>[2x]GSHMDSKHQCVKLNDGHFMPVLGFGTYAPPEVP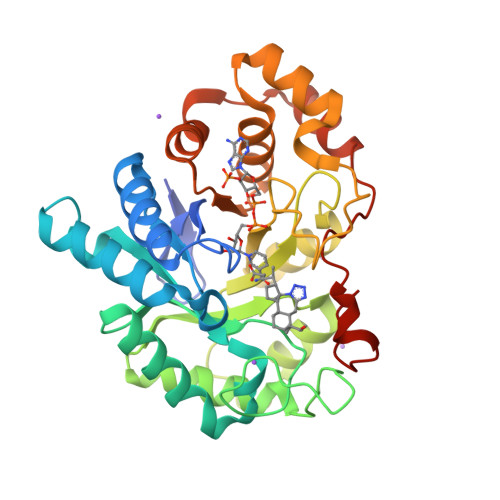RSKALEVTKLAIEAGFRHIDSAHLYNNEEQVGLAIRSKIADGSVKREDIFYTSKLWSTFHRPELVRPALENSLKKAQLDYVDLYLIHSPMSLKPGEELSPTDENGKVIFDIVDLCTTWEAMEKCKDAGLAKSIGVSNFNRRQLEMILNKPGLKYKPVCNQVECHPYFNRSKLLDFCKSKDIVLVAYSALGSQRDKRWVDPNSPVLLEDPVLCALAKKHKRTPALIALRYQLQRGVVVLAKSYNEQRIRQNVQVFEFQLTAEDMKAIDGLDRNLHYFNSDSFASHPNYPYSDEY> MQPSSSFLPDVWMAVTREPHIPEITPLSRILAAAAISTYSRQVEYDLDTGCKKKRTAPPPSPPPPSSPPPSPRLTLANAAAMTTTILRTNYALLLFYVREKYWHHAEEVCLSVIQSTDDHMFRVWRALTLERQGMANDAIREYKAVESRRTTAVPALMGMQLIYKHNRDQEGVAQTEAKLDGFEIAANMGGWVQAAALCWAMGDINAARDILLRFTDNEAAMAYRDEYTNYGTIRGWVDLLSGRGALLEKAGALFTSVMDMEEAQYSYFQADNESGSGSRGTTKWIDLNAALGYVAFLERKTQLAKAQSLLDRLFVLYPNCSIPPLVGKARLLMQAEDWEQAIEVTHRILAHDKSNVEALALEALYAMAKDTRHDAAPVRVRRLLDAVRAKEPRNVALLHQFALVFSRLAGDRLDLLSLTTQFSDMAYALDSRNGDVLCGLGYQQLYRHDDKAATETFRKAATLTDSLDPLLGTVTCLLRQGDMEAAATQLQLCNQLQPAAQRNAELSMLNAQLRWHRRGMEEETAVLRYLDQAAEAIKQDVKERAGVGMEVYVHLNAPVALAIAHAYIMHCRNEPPDPMFKHADVVGEKCGRHLEFIVQHLPACMEAQLMLAKVWFVTGEVRKAQNLLKSTLIVQEQPLPDAFLLSSQICQYMGDTKLACQALAQARTLDFSLQEKPLYNLLLGTVKGTTGEYAEALASLQRAYNTVKSAATAPSAGKPTNPLSVPETVTLYLQLAQAQLRVRDVDAARETLTEAALKFRGSAQIGRVIIAQAMLAARTDVDKSIELLRQVSSKSEFYIAAHSQLGKLFLTHKHNVAMYIQCFQEMAESVPSAQSYVELGEAYTTIQEPEQAIAAYEKAKALSPSSSELSVRVGRALVAAHD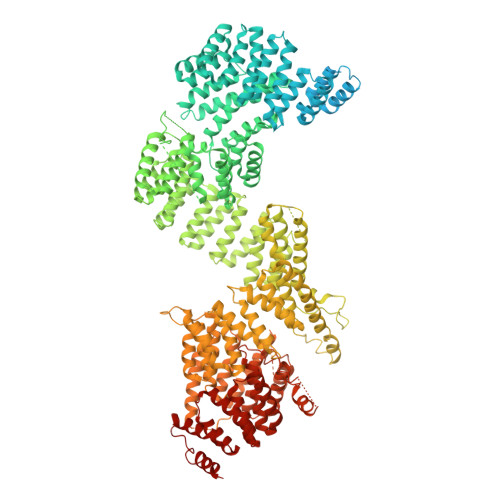YAKAIRYYQDALVTDPHLSIVRADLATLQWRLGHIEEARETIVASPVYELPSTDGAGAGVASAAAAGSAEAVGTAIERINLYLLLYKVLRDQPWTVPLSEEGTAAADSDDNHGDAALTALLTARSLQRRLLEHQLRTTEAPEVITEQRVVMSRICTEAGARCIYSTPAPPPFSVVMTDKKVEAAAALAVQSAIASRLTNAREYLREAIAFDESNERAQLESAQLCYRTGDTEGCEQHCTTVLRMAEGSANTADAAILLANLYTEQNRDEDARNMFEDLLRKTPQHYEALVYYLILLYHAGQLPEAKEALERAAAAVPIGQRADPGLSYVRGLYEHLCNNNAEALRHFNLARLPAGNPWCTRALVRMIRIYLVPTTQDLWVRGTSPAAAAATAVADPPRAKEQQQKSATPGKVPLAAATTGSTELHDNIRHAEQLLLLLPVHSEERRILQAYCTMATRRPEELETALHLFLECIVAAETGGVSAAMTAEKNGGSGSPKKTAAEERKQPRRGKGGDSDDDEDLQLLASMHEAAAELAQRSSGNSTATLAFALQCKVIHPEAFLGLAICLFISGQETAARNVLARLLESKDITTKMSAMKQAEDKEDAASKDAASKEAAEPAAPMVLSPPIAILTCSEDDTIERAMLFEAYMDTQEGRLKDARFVLQQVLSANEGCSSAWNELGLIYERNQKHKNASQCYQKAWKLVQEADPDVGYKLGFNYLRGGQPVKAIDVCKRVLTHHATYPRIEADIMDAAYSMLRP N-cyclopentylmethanesulfonamide 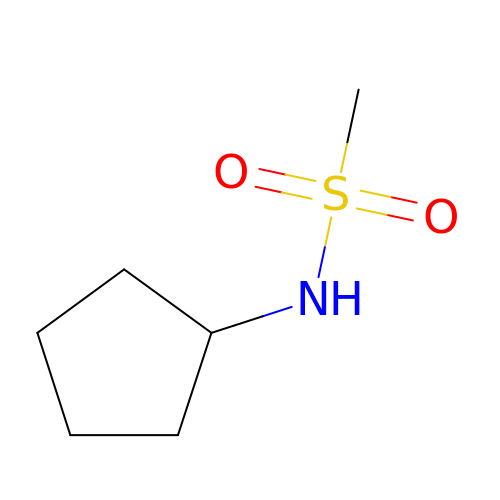| C6 H13 N O2 S | IJXUJLYIQLLJEP-UHFFFAOYSA-N> MKTITLYLDPASLPALNQLMDFTQNNEDKTHPRIFGLSRFKIPDNIITQYQNIHFVELKDNRPTEALFTILDQYPGNIELNIH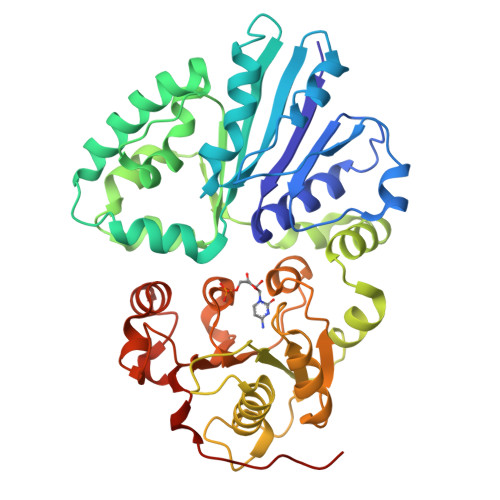LNIAHSVQLIRPILAYRFKHLDRVSIQQLNLYDNGSMEYVDLEKEENKDISAEIKQAEKQLSHYLLTGKIKFDNPTIARYVWQSAFPVKYHFLSTDYFEKAEFLQPLKEYLAENYQKMDWTAYQQLTPEQQAFYLTLVGFNDEVKQSLEVQQAKFIFTGTTTWEGNTDVREYYAQQQLNLLNHFTQAEGDLFIGDHYKIYFKGHPRGGEINDYILNNAKNITNIPANISFEVLMMTGLLPDKVGGVASSLYFSLPKEKISHIIFTSNKQVKSKEDALNNPYVKVMRRLGIIDESQVIFWDSLKQLGGGLEHHHHHH> MDIVFAADDNYAAYLCVAAKSVEAAHPDTEIRFHVLDAGISEANRAAVAANLRGGGGNIRFIDVNPEDFAGFPLNIRHISITTYARLKLGEYIADCDKVLYLDIDVLVRDSLTPLWDTDLGDNWLGACIDLFVERQEGYKQKIGMADGEYYFNAGVLLINLKKWRRHDIFKMSCEWVEQYKDVMQYQDEDILNGLFKGGVCYANSRFNFMPTNYAFMANRFASRHTDPLYRDRTNTVMPVAVSHYCGPAKPWHRDCTAWGAERFTELAGSLTTVPEEW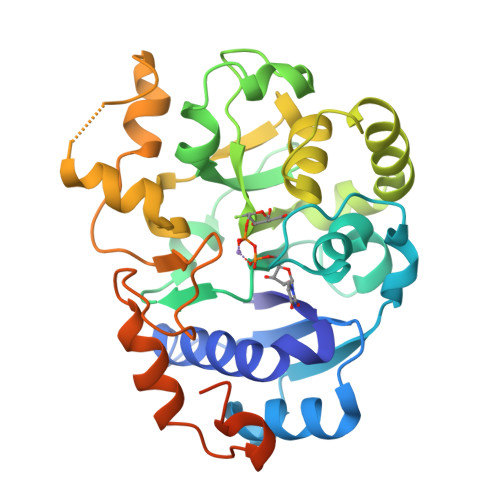RGKLAVPHRMFSTKRMLQRWRRKLSARFLRKIY>[3x]MVSRYVPDMGDLIWVDFDPTKGSEQAGHRPAV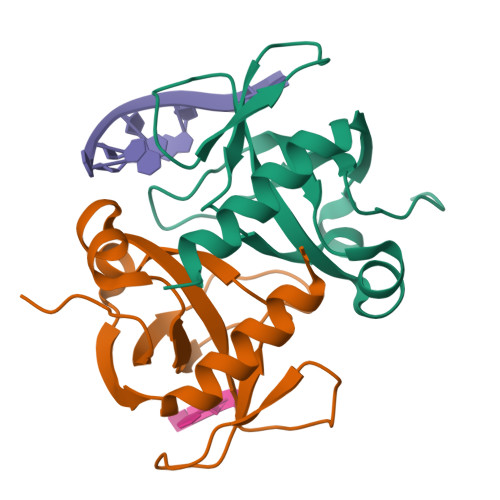VLSPFMYNNKTGMCLCVPCTTQSKGYPFEVVLSGQERDGVALADQVKSIAWRARGATKKGTVAPEELQLIKAKINVLIGHHHHHH> XMHLNPAEKEKLQIFLASELLLRRKARGLKLNYPEAVAIITSFIMEGARDGKTVAMLMEEGKHVLTRDDVMEGVPEMI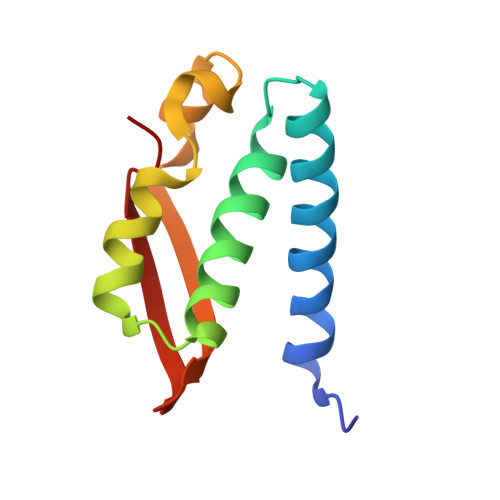DDIQAEATFPDGTKLVTVHNPIS>HHGIRMTRISREMMKELLSVYFIMGSNNTKADPVTVVQKALKGGATLYQFREKGGDALTGEARIKFAEKAQAACREAGVPFIVNDDVELALNLKADGIHIGQEDANAKEVRAAIGDMILGVSAHTMSEVKQAEEDGADYVGLGPIYPTETKKDTRAVQGVSLIEA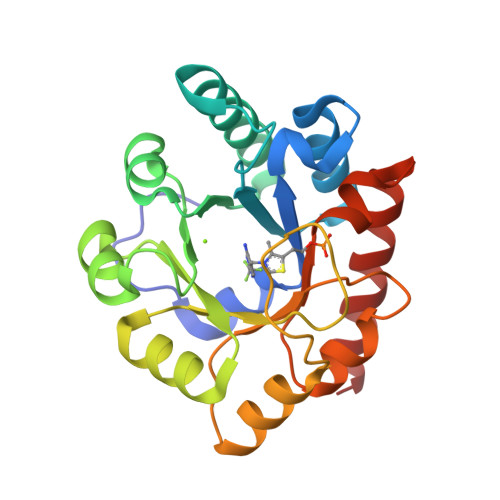VRRQGISIPIVGIGGITIDNAAPVIQAGADGVSMISAISQAEDPESAARKFREEIQTYKTGR[2x]> EKQTAKRNRREEILQSLALMLESSDGSQRITTAKLAASVGVSEAALYRHFPSKTRMFDSLIEFIEDSLITRINLILKDEKDTTARLRLIVLL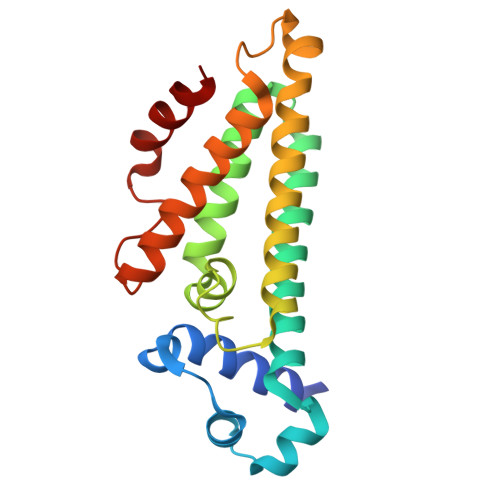ILGFGERNPGLTRILTGHALMFEQDRLQGRINQLFERIEAQLRQVMREKKMREGEGYTLDETLLASQLLAFCEGMLSRFVRSEFKYRPTDDFDARWPLVAAQLQ> KIPNFVVPGKCASVDRNKLWAEQTPNRNSYAGVWYQFALTNNPYQLIEKCVRNEYSFDGKQFVIKSTGIAYDGNLLKRNGKLYPNPFGEPHLSIDYENSFAAPLVILETDYSNYACLYSCIDYNFGYHSDFSFIFS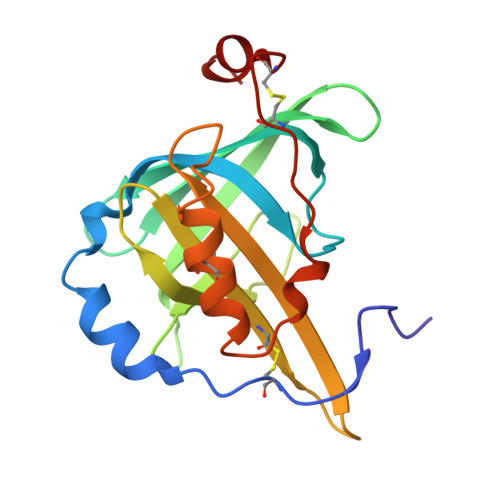RSANLADQYVKKCEAAFKNINVDTTRFVKTVQGSSCPYDTQKTV>[2x]MKSNGCRYGTHRVIEPKGVLPQPAKILNNDMSEIWDNEMLIDVIRLNIDSASFHQIKNKLIAQGHQDLEKAFAEHAIELTNRTGKHKNEDTGSGGMFIGRV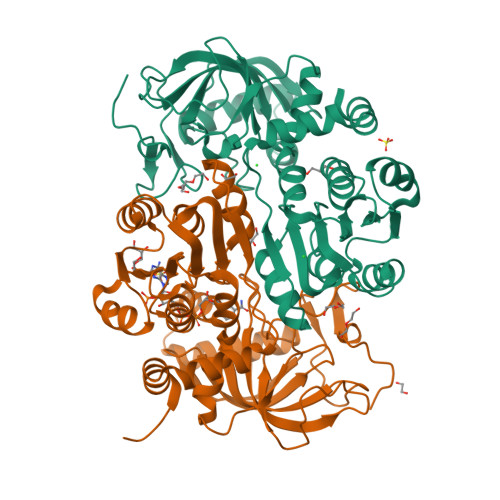AAIGDKFEMKEEVKVGDKIASLVSLSLTPLKINKVKKVLLDKDQMEIEGQAILFSSGVYAKLPDDLDENLALSVLDVAGAPAQVERLVKPDDTVVIIGANGKSGILCNAVAKERAGICGKVIGVVRNENYIPTCKATGCDEVILAQATDAITIQKEVSRLTNGKMADVVINVVNTEDTELPSIMAAKDRGMVYFFSMATSFTKAALGAGGIGYDVDMMIGNGYAHHHSEIALDLLRRNSVLMKIFKERYAEHHHHHH>[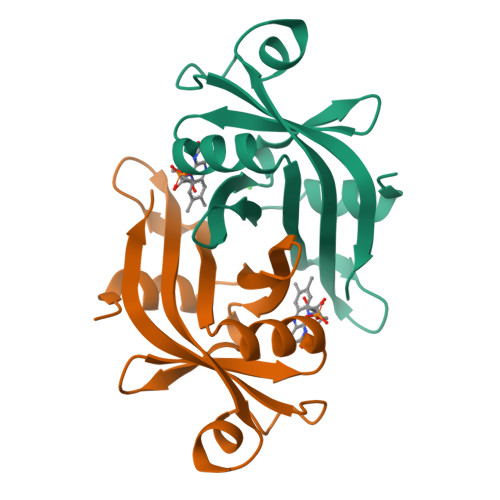4x]MLPGTFFEVLKNQGVVAIATQGEDGPHLVNTWNSYLKVLDGNRIVVPVGGMHKTEANVARDERVLMTLGSRKVAGRNGPGTGFLIRGSAAFRTDGPEFEAIARFKWARAALVITVVSAEQTL>GGADKLPNIVILATGGTIAGSAATGTQTTGYKAGALGVDTLINAVPEVKKLANVKGEQFSNMASENMTGDVVLKLSQRVNELLARDDVDGVVITHGTDTVEESAYFLHLTVKSDKPVVFVAAMRPATAISADGPMNLLEAVRVAGDKQSRGRGVMVVINDRIGSARYITKTNASTLDTFRANEEGYLGVIIGNRIYYQNRIDKLHTTRSVFDVRGLTSLPKVDILYGYQDDPEYLYDAAIQHGVKGIVYAGMGAGSVSVRGIAGMRKALEKGVVVMRSTRTGNGIVPPDEELPGLVSDSLNPAHARILLMLALTRTSDPKVIQEYFHT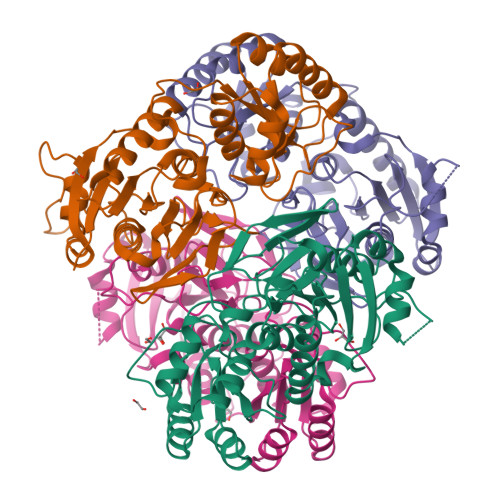Y[4x]>SFTSSGMECKNPDSLHVFLVSAPGQGNVTPMLRLAKSLASKGLLVTFSTPESYGKEMRKTNDDISDQPILIGEGSIRFEFLDDEWDENEHKGEGLDAYATHLERVGKQNLPRMFKKHEEEGRPISCIINNPFIPWVPEVAESLGIPSALLWVQSCASFSSYYHFFNDLVSFPTESNLKKDVCLPSMPMLKYDEVPLLLYPIVPLPIISLKNAMLRQQKNLSKTFCVLVDTFQQLEDELIHYLSKLCPIRPIGPLFKISDTSSSNISGD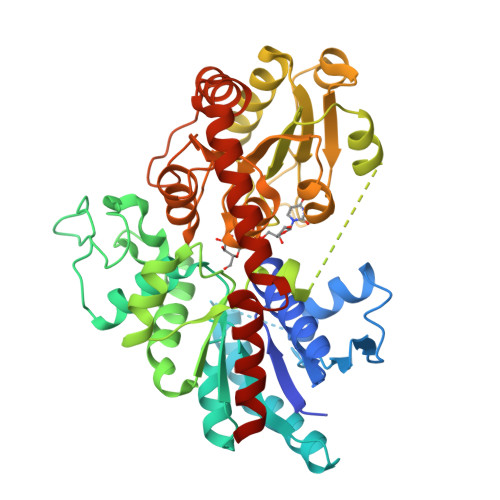IRKADDCIEWLDSKSPSSVVYISFGSIVHLKQEQITEIAYALMNINISFLWVMKPPQKDSYDKQHVLPQGFLEKVGEKGKVVKWSPQEQVLSHQSLACFVTHCGWNSSMEALANGIRVVTLPQWGDQVTNAKFLVDVFGVGVRLSRGDLEDRIIPREEIELRLLEVTSGEKATEMKHNALRWKKAAEEAVAKDGSSSKNLQEFVDELNNFRFIT[2x]>[2x]MGSPKNLLVRLRSNMEPFSKKLRVVADYILENAHDVQFQTITDLARNTQTSEA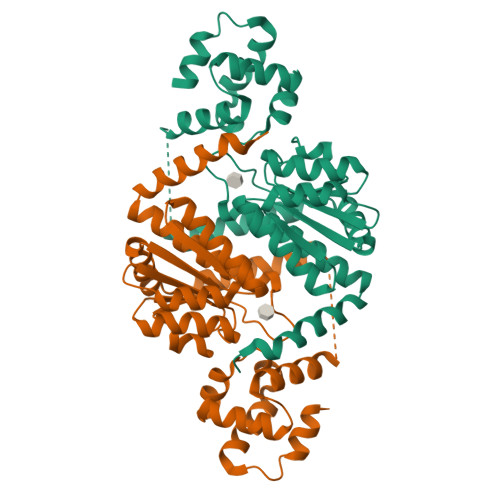TVVRLCRDMGYKGYSDFRMALAVDLSQTESRQQNHIEGDICDVSAQSAVDSLQDTAKLIDRKSLARIVERVHQAEFIGCIGVGASSIVGRYLAYRLIRIGKKAIMFEDTHLAAMSASRSSQGDLWFAVSSSGSTKEVIHAAGLAYKRDIPVVSLTNINHSPLSSLSTEMLVAARPEGPLTGGAFASKVGALLLVDVLVNSLLESYPEYKDSVQETAEVVIPLMAN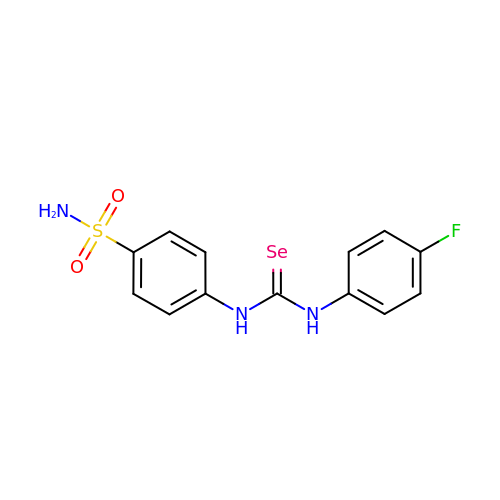1-(4-fluorophenyl)-3-(4-sulfamoylphenyl)selenourea | C13 H12 F N3 O2 S Se | WEUISFFZQUMPMK-UHFFFAOYSA-N>[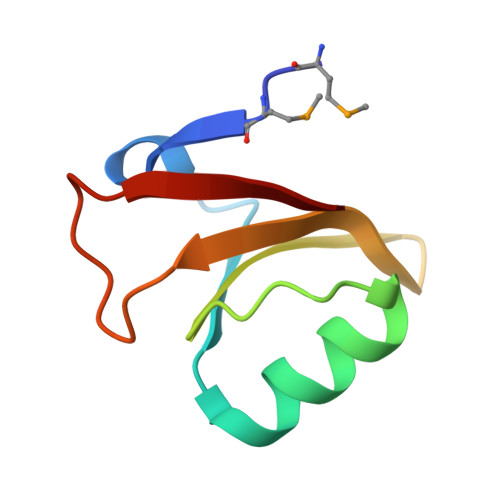4x]MKMRKLVKDFGDDYTLIQDSQEVKAILEYIGSEEEPHALFVKVGDGDYEEVWGIDSFVPYNFLEAYRLK>[2x]MTQAWLWIGVISMALGSVFFGFGAHN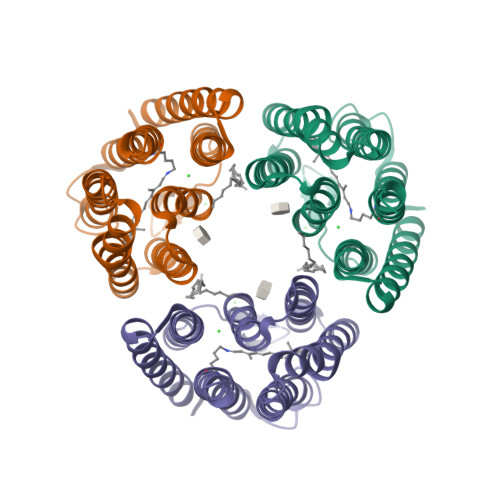AKNERWQILYTLNFFICLIAAGLYLAMALGLGVNVINGRPTYWVRFVTWFCSTPLLLLDLTFLGRTSLPLTGSLLGANAYMLVTGFVATVTPKPMSYIWYIVSCAAYLAIVYLLAQPYRIAAERKHPRSKQAFRTLVTVHLVLWTLYPIVWILSPEGFSTFTQGSETMFYTLLDIASKVGFGFLSLNTLHTLEQATEPARETHLSYLEHHHHHH>TMTSVGVRALRQQASELLRRVEAGETIEITDRG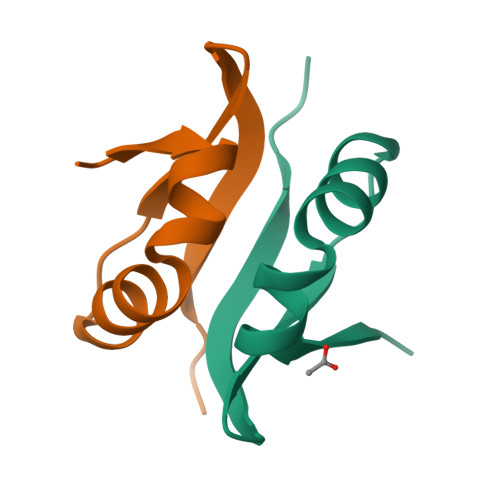RPVALLSPLPQ[4x]>MCNSCEKELETKFPADKIDLTLLEPVFKEYAGKAGSIIGILQKTQEIYGYLPLAALQAIADNTDNKRAKIYGIATFYSQFRLNPVGKYVILQCQGTACHVLGSKAIGSAICDELGITPGQTTADGLFTLEDVACLGCCSLAPVIMINGEAYGKLTPTSVRKILQDIAEAEKGGVVSEG[4x];>[4x]MKVRVGLGSCGIAAGGRKVMDRLAQEIKNHGKEIELLPTGCIGMCFYEPIVDVFDGDKVYSYANVTADMATEIFNSHIIGGQPLTQYIVSTTEKPYTILAKQVRIALRNCGVIDPENVDEYKANDGYKALSKALKEMTPEEVIEEIKVAGLRGRGGAGFPTWFKWNAARQSKGEIKYVVCNADEGDPGAFMDRSVLEGDPHALLEGMAICGYAIGANEGHIYCRAEYPLAIKRLEIAIADAKQRNLLGKNIMGTNFSFDMKIKKGAGAFVCGEETALIASLEGERGMPRLKPPFPAQSGFWGKPTNINNVETFANVPWIMYNGGSAYAAYGTEKSKGTKVFALAGKIKNGGLVEVPMGMSLREVIYDIGGGILNDREFKAVQMGGPSGGCIPKQLLDTPVDYDSINKTGAIMGSGGMIVMDETTCMVDMARFFLDFTVKESCGKCIYCRIGTKRMLEILERITTGEGREGDIEELEELSISIKDGSLCGLGQTAPNPVLTTIRYFRDEYEAHIRDKKCPAKSCKPLLTYTINQDNCKGCTLCAQKCPVQAITGEKKKPHVIDQALCTKCGNCASVCRLDAVCIE;>MSKISININGRELVVSAGQTILQAAAEHGIEIPHLCHDERIQPYGACGLCVVEVEGSPKLVRSCATSVQNGQVIRTDTSRTVVARKTALQLLASDHRGDCRPPCMLACPAQTDCQGYVGLIANGQYEEALKLIKDKMPIPASIGKICPHPCETACRRELVEEPISIAQLKSFVAEVDLNGNQYQPPMKPATGKKVAVVGAGPAGLTAAYFLARDGHKVVIYEAMPHPGGMLRYGIPQYRLDKALLDAEVALMTKMGIEIIYNTKIGDDVSLDYLHDNYDAVFLGIGSWQSQGLRCKGEDMEGVLGGIDFLREVTMNSNITLGGKVLVVGGGNTAMDVARTSKRLGAEEVTIIYRRTIDEMPAEKIEIHEAQEEGVKFQLLVAPVEVLGENGHAKALKCEIMRLGEPDASGRRKPEPTGETVVYEADRIIAAIGQKTVIGNIKDIATDKSGNIIVNGGAFTTNRDKVFAGGDAVTGPKIAIDAIAQGKNAAQVIDSYLNGCLVPHADSQYFTQKDITAADLADRAKAPRVSLTVEDAEVRNKSFMQVAKTFTEEEALRESKRCLECGCRDYFECQLIKYIQDYDVSTEKDSQVECHKTTEFDNHPFIERNPDKCVLCGLCVRVCDEVVGATAIGLVGRGFDSVIMPEFKLPLSETACISCGQCVDVCPTGACMEKQVSYKQIPANMDSMASVCGYCGVGCNVNIEYKGDVVFRVTPDRVNDDGWLCQRGKFGLGHANDKARLTAPVIKRNGQFVKVDWNEANLEVVKRLQAVVAAYGKDSIGVVVSPRLTNEELFLAGKLADAVNTTIKTSYSVDGGSGLGSVLGYDASTNSFAELDNSDFVLTLGKVKENHPVLDFKIRLSGVCSVAWPQSLANTADMKVFLKALLNLGVDENKVAEKTEGFAELKASLADVKVSEEIQALAQKYAKAAKPLIVIDEDTVSAEAVKLMAYAAVITGKIGAAYRGIILVRTKNNTQGAVDMGFVMPVSAVAQGIESGKIKALVVIGEDPAAYPQESALLQKLSFLVVYDMFMTKTATAADMVVPLVSSAEVNGTYTRSDRRIQAVRAAIQPKTGKATLQILIETLKSLGIKYDTIADVRAAIASEVSNYAGMDAADFGTTVYWPNNKNVLYTDGFATEGQKAILAAVGDVPVFVEKKKYDSVEMNFVNGRQSL[4x]

Here, we present the single-particle cryo-EM structure of the Stn family transhydrogenase from the acetogenic bacterium Sporomusa ovata and functionally dissect its electron transfer pathway. Stn forms a tetramer consisting of functional heterotrimeric StnABC complexes. Our findings demonstrate that the StnAB subunits assume the structural and functional role of a bifurcating module, homologous to the HydBC core of the electron-bifurcating HydABC complex. Moreover, StnC contains a NuoG-like domain and a GltD-like NADPH binding domain that resembles the NfnB subunit of the NfnAB complex.

One state is the isolated or purified state of the enzyme in the absence of any added substrates (NADPH, NAD+, and Fd) and cofactor (FMN), referred to as StnABCS1 state hereafter. After 2D classification, the best particles were used for 3D reconstruction with applied D2 symmetry, where they were refined to obtain a global resolution of 3.2 Å for the StnABCS1 and 3.0 Å for the StnABCS2 state of the complex. In the structure of the StnABCS1 state, only FAD was present in the StnC subunit but no FMN could be observed in the binding cavity of the StnB subunit. As expected, the StnABCS1 state of the enzyme was found to contain only FAD in StnC subunit, whereas the StnB subunit lacked an FMN despite being homologous to the HydB from the HydABC complex. We reasoned that FMN is only loosely bound in StnB and only a fraction of the protein complex harboured FMN during the protein purification. Therefore, the electron density for FMN was averaged out within the density for the StnABCS1 structure. The [4Fe4S]-cluster C7 next to FAD has an unusual ligand sphere where three cysteine residues along with a lysine residue (K170) seem to coordinate the metals in the [4Fe4S]-cluster in the StnABCS1 state of the enzyme. In StnC we now observe in our structure that either a lysine or a cysteine residue coordinates the proximal [4Fe4S]-cluster in the StnABCS1 or StnABCS2 state, respectively. However, they differ in the occupancy of substrates and cofactors.>EWQENKSWNAHFTEHKSQGVVVLWNENKQQGFTNNLKRANQAFLPASTFKIPNSLIALDLGVVKDEHQVFKWDGQTRDIATWNRDHNLITAMKYSVVPVYQEFARQIGEARMSKMLHAFDYGNEDISGNVDSFWLDGGIRISATEQISFLRKLYHNKLHVSERSQRIVKQAMLTEANGDYIIRAKTGYSTRIEPK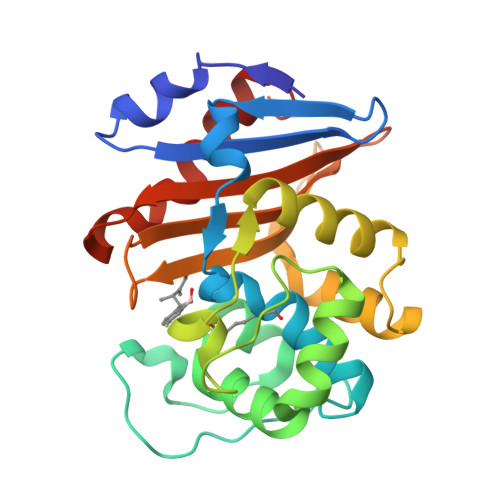IGWWVGWVELDDNVWFFAMNMDMPTSDGLGLRQAITKEVLKQEKIIP[4x]>[2x]MCLPTIRKIAIIGAGPSGLVTAKALLAEKAFDQVTLFERRGSPGGVWNYTSTLSNKLPVPSTNPILTTEPIVGPAALPVYPSPLYRDLQTNTPIELMGYCDQSFKPQTLQFPHRHTIQEYQRIYAQPLLPFIKLATDVLDIEKKDGSWVVTYKGTKAGSPISKDIFDAVSICNGHYEVPYIPNIKGLDEYAKAVPGSVLHSSLFREPELFVGESVLVVGGASSANDLVRHLTPVAKHPIYQSLLGGGDI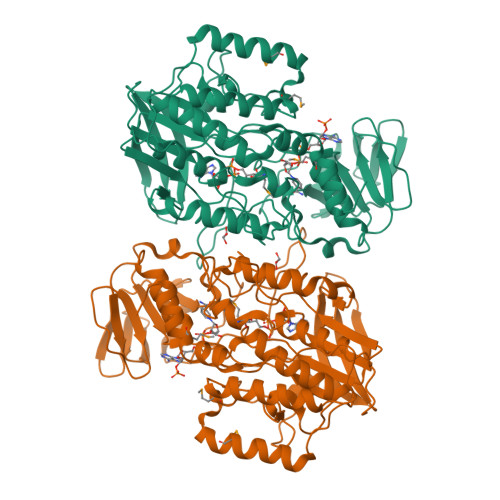QNESLQQVPEITKFDPTTREIYLKGGKVLSNIDRVIYCTGYLYSVPFPSLAKLKSPETKLIDDGSHVHNVYQHIFYIPDPTLAFVGLALHVVPFPTSQAQAAFLARVWSGRLKLPSKEEQLKWQDELMFSLSGANNMYHSLDYPKDATYINKLHDWCKQATPVLEEEFPSPYWGEKERSIRENMWSIRAKFFGIEPPK> MSILEKITSSPSECAEHITNKDSCLSKKIQKELTSFLQKKETLGCDSESCVITHPAVKAYAQQKGLDLSKELETRFKAPGPRNNTGLLTNFNIDETLQRWAIKYTKFFNCPFSMMDFERIHYKFNQVDMVKVYKGEELQYVEGKAVKRPCNTFGCVLNTDF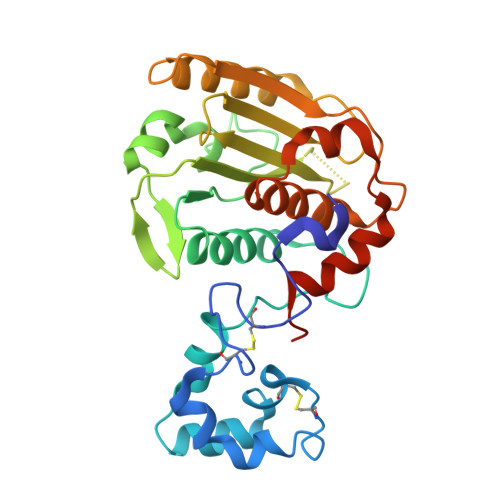STGTGKHWVAIFVDMRGDCWSIEYFNSAGNSPPGPVIRWMERVKQQLLKIHHTVKTLAVTNIRHQRSQTECGPYSLFYIRARLDNVSYTHFISTRITDEEMYKFRTHLFRIALEHHHHHH>[4x]MSMDISDFYQTFFDEADELLADMEQHLLDLVPESPDAEQLNAIFRAAH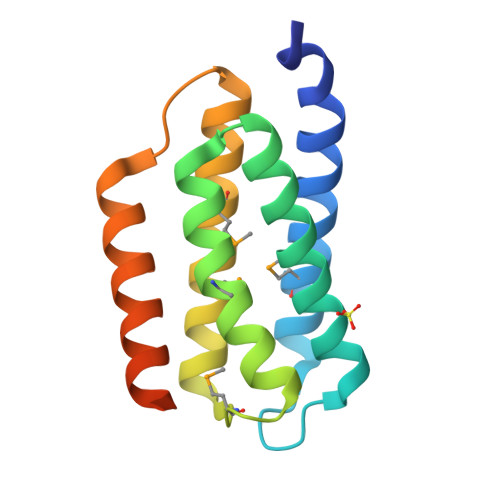SIKGGAGTFGFTILQETTHLMENLLDEARRGEMQLNTDIINLFLETKDIMQEQLDAYKNSEEPDAASFEYICNALRQLALEAKGETTPAVRSHHHHHH3-{(2Z,3S,4S)-5-[(Z)-(4-ethenyl-3-methyl-5-oxo-1,5-dihydro-2H-pyrrol-2-ylidene)methyl]-2-[(5R)-2-[(3-ethyl-5-formyl-4-methyl-1H-pyrrol-2-yl)methyl]-5-(methoxycarbonyl)-3-methyl-4-oxo-4,5-dihydrocyclopenta[b]pyrrol-6(1H)-ylidene]-4-methyl-3,4-dihydro-2H-pyrrol-3-yl}propanoic 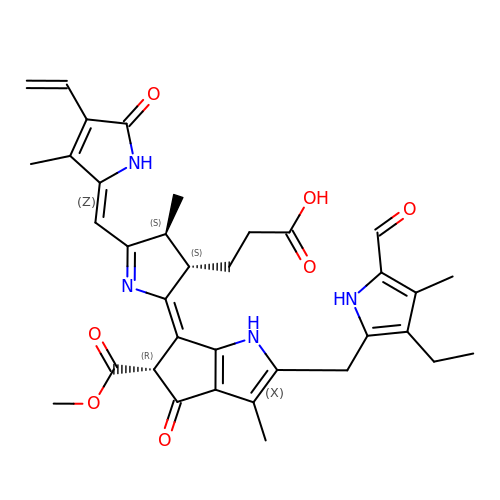acid | C35 H38 N4 O7 | ZDEZVOKVUGXDCZ-FATBKOMMSA-N>[3x]SNA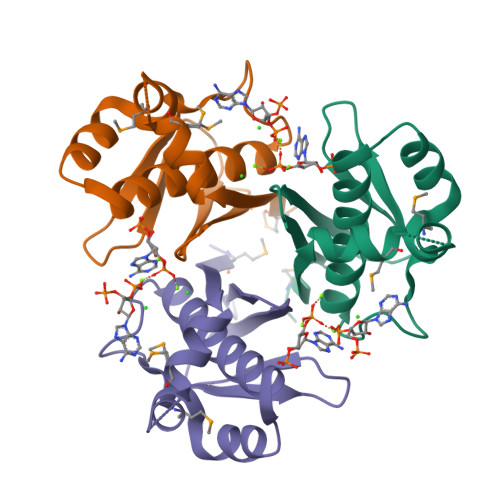MIVGIGIDIIELNRIEKMLDGKLKFMERILTENERNVAKGLKGSRLTEFVAGRFAAKEAYSKAVGTGIGKEVSFLDIEVRNDDRGKPILITSTEHIVHLSISHSKEFAVAQVVLESSSS> MTQSNAAPHSHAANAS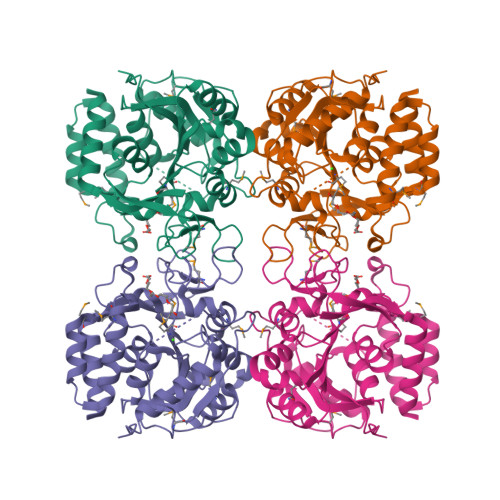PKAIRPLASATPIILDCDPGHDDAISLILALSSERLNPLAVTTSAGNQTPDKTLNNALRILTLLNRADMPVAGGAVKPLARELIIADNVHGESGLDGPKLPDPSFDPLTQNAIELMAEKVRQSAVPVTLVPSGPLTNIALFIANYPELHSKVERIVLMGGAAGVGNWTPAAEFNIFVDPEAADMVFKSGIPITMCGLDVTHEAQIMDEDIERIRAIPNPVAQCVAELLDFFMIYHRDPKWGFTGAPLHDPCTIAWLLKPELFTAQECWVGVETKGEYTQGMTVVDRYQLTGKTANATVLFDLDRQGFVDLIVDCLSAYN>SMNAVQEIMIPASKAGLVIGKGGETIKQLQERAGVKMVMIQDG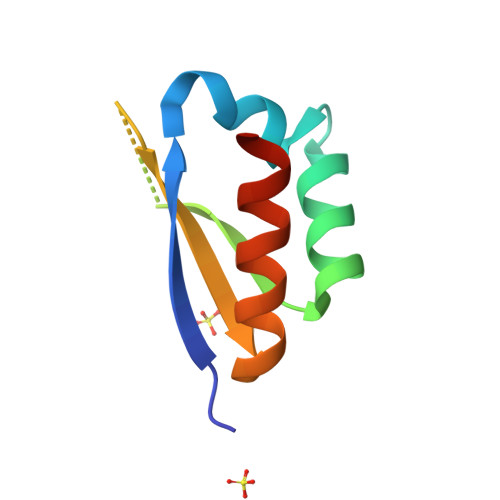PQNTGADKPLRITGDPYKVQQAKEMVLELIRDQG[4x]> M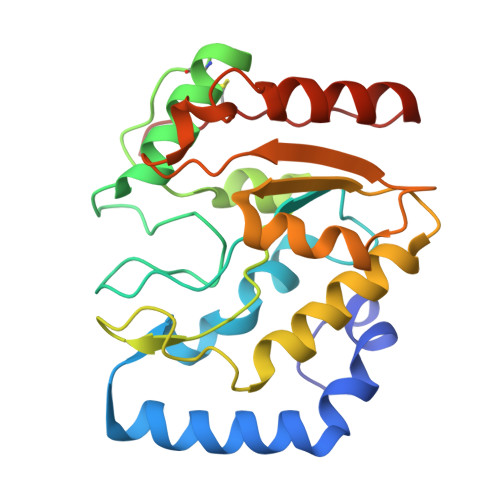KQLLQDSWWNQLKEEFEKPYYQELREMLKREYAEQTIYPDSRDIFNALHYTSYDDVKVVILGQDPYHGPGQAQGLSFSVKPGVKQPPSLKNIFLELQQDIGCSIPNHGSLVSWAKQGVLLLNTVLTVRRGQANSHKGKGWERLTDRIIDVLSERERPVIFILWGRHAQMKKERIDTSKHFIIESTHPSPFSARNGFFGSRPFSRANAYLEKMGEAPIDWCIKDL> SMPKTISVRVTTMDAELEFAIQPNTTGKQLFDQVVKTIGLREVWFFGLQYQDTKGFSTWLKLNKKVTAQDVRKESPLLFKFRAKFYPEDVSEELIQDITQRLFFLQVKEGILNDDIYCPPETAVLLASYAVQSKYGDFNKEVHKSGYLAGDKLLPQRVLEQHKLNKDQWEERI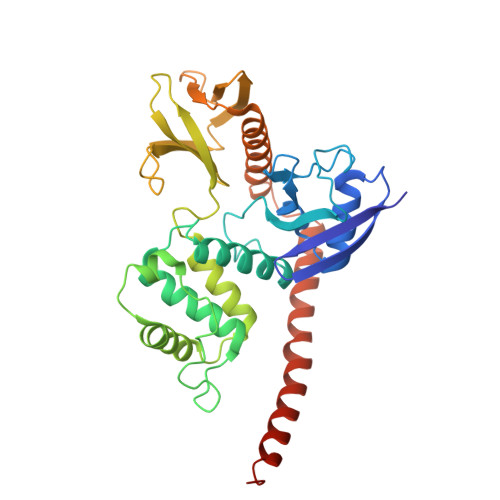QVWHEEHRGMLREDAVLEYLKIAQDLEMYGVNYFSIKNKKGSELWLGVDALGLNIYEQNDRLTPKIGFPWSEIRNISFNDKKFVIKPIDKKAPDFVFYAPRLRINKRILALCMGNAELYMRRRKPDTIEVQQMKAQAREEKHQKQMERAMLENEKKKREMAEKEKEKIEREKEE N-{4-[amino(dihydroxy)-lambda~4~-sulfanyl]-2-methylphenyl}-2-(4-chloro-2-{[3-fluoro-5-(trifluoromethyl)phenyl]carbonyl}phenoxy)acetamide 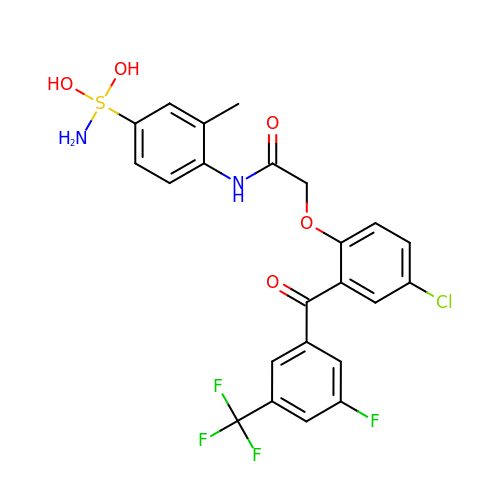| C23 H19 Cl F4 N2 O5 S | RXLXGVALXIAUEE-UHFFFAOYSA-N> SHMSLIRGVVVSKQLVYDPTGTKYVKIDVVEEKELPGPVAAFSAQDEQAAQLMREVMPLVTQIVRSLPFGGGKITVPRITLWLTEEEEEVFGDIDVGDVIEINIENGAITIKPES

The similarity of eukaryotic actin to crenactin, a filament-forming protein from the crenarchaeon Pyrobaculum calidifontis supports the theory of a common origin of Crenarchaea and Eukaryotes. Attempts to trace back the origins of today's eukaryotic F-actin filaments led to the discovery of crenactin found in certain organisms of the order Thermoproteales within the phylum Crenarchaeota (Crenarchaea, part of the 'TACK' superphylum). Hence, it has been proposed that crenactin filaments share a common ancestor with F-actin. In Pyrobaculum calidifontis, crenactin is encoded within the arcade cluster of genes, together with four arcadins, and has been proposed to be part of a cell-shape maintenance system.

In addition, we show that crenactin interacts with two of the arcadins, arcadin-1 and arcadin-2.> MQKRTLYN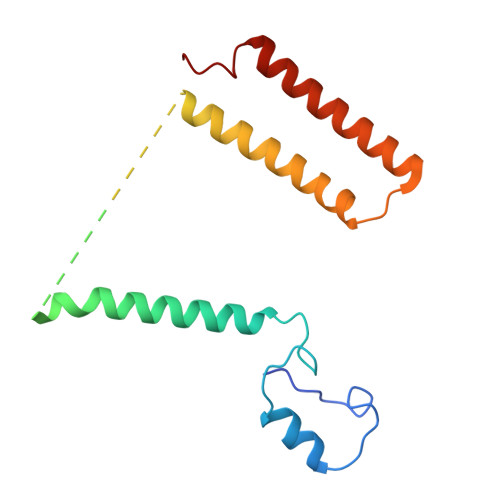AMTPAQRYFVEGEHVVQAEANRDILFTQLDSNSYLPVLHYVLVGTALGVVFLVLPLLIAPARVDLDKISAYECGFDAFGEARETFSVSFYIVSIMYLLFDIEVVYLIPYVMTNATEYMYWVMQTFVAILVGGFFYEWRMGALEWRE> EFPHNAIEPCVICQTRPKNGCIVHGKTGHLMACFTCAKKLKKRNKPCPVCRQPIQMIVLTYFP;>[2x]EIVEPEFPHNAIEPCVICQTRPKNGCIVHGKTGHLMACFTCAKKLKKRNKPCPVCRQPIQMIVLTYFP;> EPEFPHNAIEPCVICQTRPKNGCIVHGKTGHLMACFTCAKKLKKRNKPCPVCRQPIQMIVLTYFP

The most prominent regulator of p53 is the Ub ligase (E3) MDM2, which binds to the transactivation domain of p53 through its N-terminal p53-binding domain, thereby inhibiting p53’s transcriptional activity. Furthermore, MDM2 catalyzes ubiquitination of p53, where monoubiquitination promotes nuclear export of p53 and polyubiquitination leads to proteasomal degradation. ATM phosphorylates MDM2 on six residues (S386, S395, S407, T419, S425, and S429) that are close to the C-terminal RING domain and far from the domains associated with p53 binding. Here, we show that S429 phosphorylation selectively enhances MDM2 homodimer E3 activity, but has no effect on MDM2-MDMX heterodimer E3 activity.

A prior solution structure of MDM2 RING domain homodimer determined by nuclear magnetic resonance showed that this region is flexible and adopts various conformations, suggesting that the 310-helical turn configuration observed in our structures might be a product of UbcH5B–Ub binding. Since flexible or disordered regions usually lack electron density in crystal structures, we also crystallized and determined the structure of cat MDM2-422–C-S429E to 1.21 Å. The asymmetric unit contains two dimers. The electron density for residues 429–C was visible and MDM2 adopts the same configuration as seen in the cat MDM2-422–C-S429E-UbcH5B–Ub structure (r.m.s. deviation of 0.30 Å for all Cα atoms). Despite contributing to crystallographic contacts, the region preceding the RING domain is able to adopt the same 310-helical turn configuration independent of E2–Ub binding. In all the structures of MDM2 homodimer bound to UbcH5B–Ub presented here, the N-terminal region preceding the MDM2 RING domain adopts the same 310-helical turn configuration.>[2x]MERPQPDSMPQDLSEALKEATKEVHTQAENAEFMRNFQKGQVTRDGFKLVMASLYHIYVALEEEIERNKESPVFAPVYFPEELHRKAAL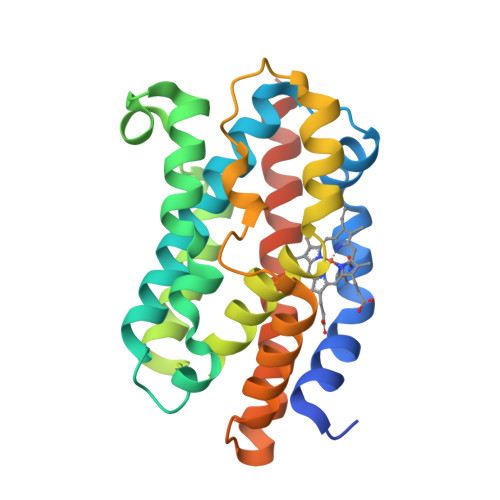EQDLAFWYGPRWQEVIPYTPAMQRYVKRLHEVGRTEPELLVAHAYTRYLGALSGGQVLKKIAQKALDLPSSGEGLAFFTFPNIASATKFKQLYRSRMNSLEMTPAVRQRVIEEAKTAFLLNIQLFEELQELLTHDTKDQSPSRA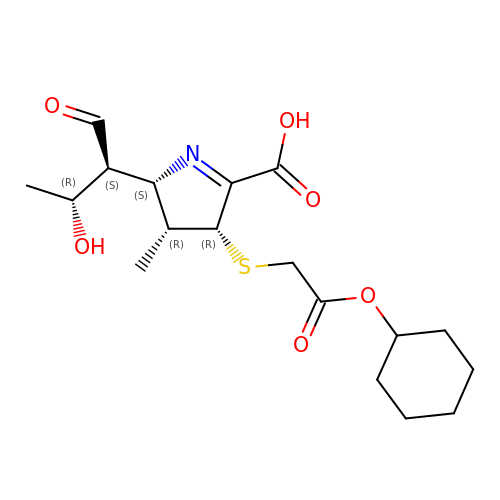(2~{S},3~{R},4~{R})-4-(2-cyclohexyloxy-2-oxidanylidene-ethyl)sulfanyl-3-methyl-2-[(2~{S},3~{R})-3-oxidanyl-1-oxidanylidene-butan-2-yl]-3,4-dihydro-2~{H}-pyrrole-5-carboxylic acid | C18 H27 N O6 S | QMGXAXLXTHMRPO-IUSQFIQGSA-N>[2x]MEKTITIYTDGAASGNPGKGGWGALLMYGSSRKEISGYDPATTNNRMELMAAIKGLEALKEPARVQLYSDS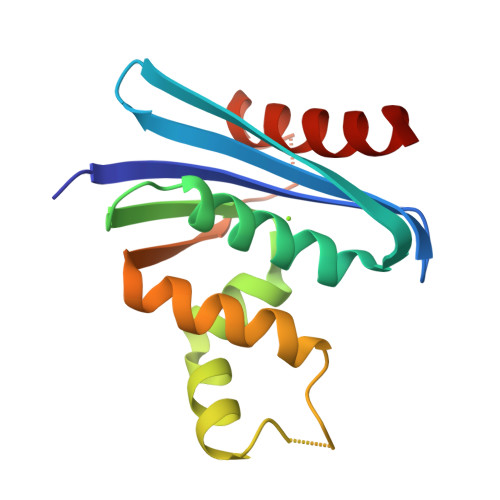AYLVNAMNEGWLKRWVKNGWKTAAKKPVENIDLWQEILKLTTLHRVTFHKVKGHSDNPYNSRADELARLAIKENS> MSSDADAHKVGLIPVTLMVSGAIMGSGVFLLPANLASTGGIAIYGWLVTIIGALGLSMVYAKMSFLDPSPGGSYAYARRCFGPFLGYQTNVLYWLACWIGNIAMVVIGVGYLSYFFP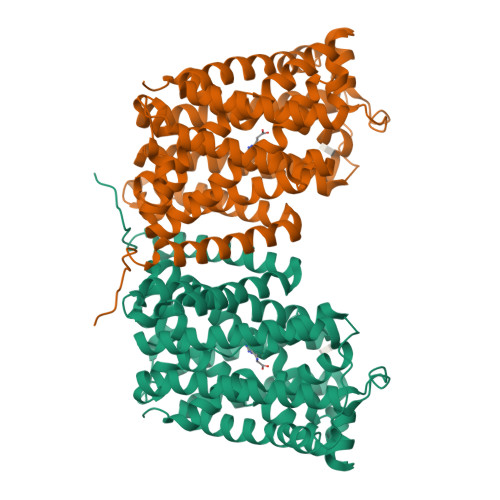ILKDPWVLTITCVVVLWIFVLLNIVGPKMITRVQAVATVLALIPIVGIAVFGWFWFRGETYMAAWNVSGLGTFGAIQSTLNVTLWSFIGVESASVAAGVVKNPKRNVPIATIGGVLIAAVCYVLSTTAIMGMIPNAALRVSASPFGDAARMALGDTAGAIVSFCAAAGCLGSLGGWTLLAGQTAKAAADDGLFPPIFARVNKAGTPVAGLIIVGILMTIFQLSSISPNATKEFGLVSSVSVIFTLVPYLYTCAALLLLGHGHFGKARPAYLAVTTIAFLYCIWAVVGSGAKEVMWSFVTLMVITAMYALNYNRLHKNPYPLDAPISKD> 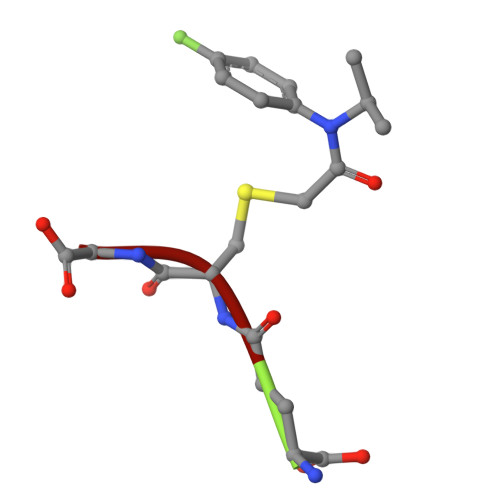ECG> AREDVVVTITETGYAKRTKTDLYRSQKRGGKGVQGAGLKQDDIVAHFFVCSTHDLILFFTTQGRVYRAKAYDLPEASRTARGQHVANLLAFQPEERIAQVIQIRGYTDAPYLVLATRNGLVKKSKLTDFDSNRSGGIVAVNLRDNDELVGAVLCSAGDDLLLVSANGQSIRFSATDEALRPMGRATSGVQGMRFNIDDRLLSLNVVREGTYLLVATSGGY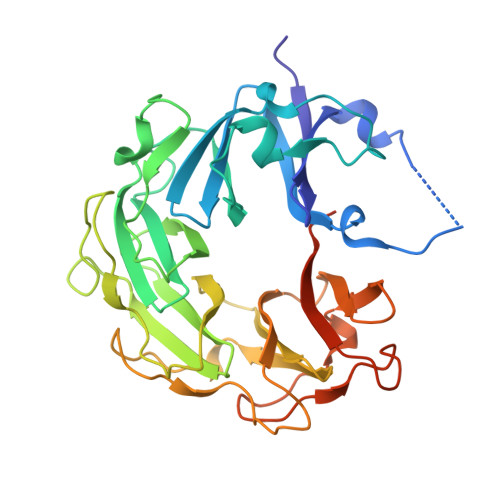AKRTAIEEYPVQGRGGKGVLTVMYDRRRGRLVGALIVDDDSELYAVTSGGGVIRTAARQVRKAGRQTKGVRLMNLGEGDTLLAIARNAEESGDDNAVDANGADQTGN> MVSFFKTPIFILIIFLYLNEKVICSINENQNENDTISQNVNQHENINQNVNDNDNIEQLKSMIGNDELHKNLTILEKLILESLEKDKLKYPLLKQGTEQLIDISKFNKKNITDADDETYIIPTVQSTFHDIVKYEHLIKEQSIEIYNSDISDKIKKKIFIVRTLKTIKLMLIPLNSYKQNNDLKSALEELNNVFTNKEAQEESSPIGDHGTFFRKLLTHVRTIKENEDIENKGETLILGDNKIDVMNSNDFFFTTNSNVKFMENLDDITNQYGLGLINHLGPHLIALGHFTVLKLALKNYKNYFEAKSIKFFSWQKILEFSMSDRFKVLDMMCDHESVYYSEKKRRKTYLKVDRSNTSMECNILEYLLHYFNKYQLEIIKTTQDTDFDLHGMMEHKYIKDYFFSFMCNDPKECIIYHTNQFKKEANEENTFPEQEEPNRQISAFNLYLNYYYFMKRYSSYGVKKTLYVHLLNLTGLLNYDTRAYVTSLYLPGYYNAVEMSFTEEKEFSKLFESLIQCIEKCHSDQARQISKDSNLLNNITKCDLCKGAFLYANMKFDEVPSMLQKFYVYLTKGLKIQKVSSLIKTLDIYQDYSNYLSHDINWYTFLFLFRLTSFKEIAKKNVAEAMYLNIKDEDTFNKTVVTNYWYPSPIKKYYTLYVRKHIPNNLVDELEKLMKSGTLEKMKKSLTFLVHVNSFLQLDFFHQLNEPPLGLPRSYPLSLVLEHKFKEWMNSSPAGFYFSNYQNPYIRKDLHDKVLSQKFEPPKMNQWNKVLKSLIECAYDMYFEQRHVKNLYKYHNIYNINNKLMLMRDSIDLYKNNFDDVLFFADIFNMRKYMTATPVYKKVKDRVYHTLHSITGNSVNFYKYGIIYGFKVNKEILKEVVDELYSIYNFNTDIFTDTSFLQTVYLLFRRIEETYRTQRRDDKISVNNVFFMNVANNYSKLNKEEREIEIHNSMASRYYAKTMFAAFQMLFSTMLSNNVDNLDKAYGLSENIQVATSTSAFLTFAYVYNGSIMDSVTNSLLPPYAKKPITQLKYGKTFVFSNYFMLASKMYDMLNYKNLSLLCEYQAVASANFYSAKKVGQFLGRKFLPITTYFLVMRISWTHAFTTGQHLISAFGSPSSTA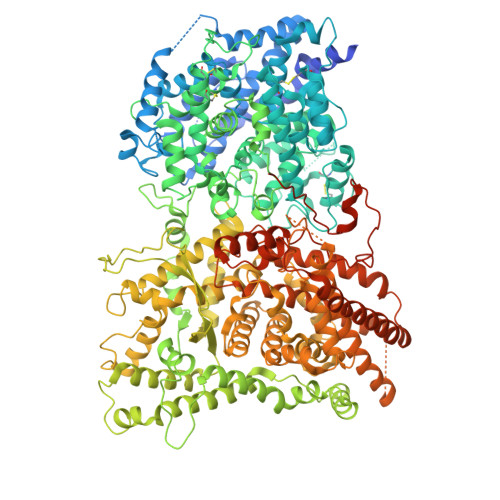NGKSNASGYKSPESFFFTHGLAAEASKYLFFYFFTNLYLDAYKSFPGGFGPAIKEQTQHVQEQTYERKPSVHSFNRNFFMELVNGFMYAFCFFAISQMYAYFENINFYITSNFRFLDRYYGVFNKYFINYAIIKLKEITSDLLIKYEREAYLSMKKYGYLGEVIAARLSPKDKIMNYVHETNEDIMSNLRRYDMENAFKNKMSTYVDDFAFFDDCGKNEQFLNERCDYCPVIEEVEETQLFTTTGDKNTNKTTEIKKQTSTYIDTEKMNEADSADSDDEKDSDTPDDELMISRFH>[11x]KQPAAEQDSSAEHADKGLHLEQQLYSVMEDICKLVDAIPLHELTSISCAK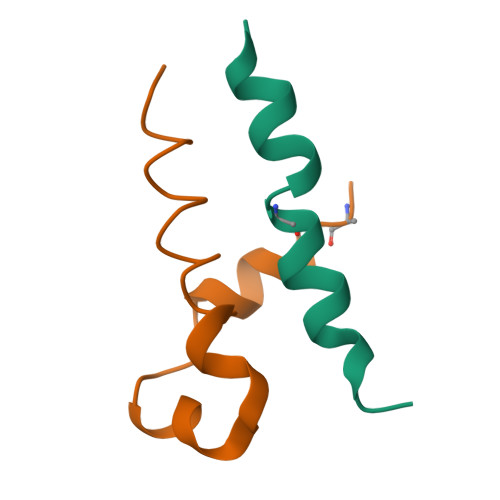ELLQQRELRRKLLADSVD>[2x]MASMKTAQE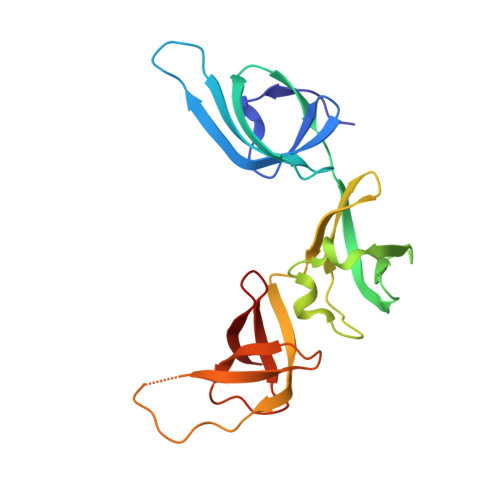FRAGQVANINGAPWVIQKAEFNKSGRNAAVVKMKLKNLLTGAGTETVFKADDKLEPIILDRKEVTYSYFADPLYVFMDSEFNQYEIEKDDLEGVLTFIEDGMTDICEAVFYNDKVISVELPTTIVRQIAYTEPAVRGDTSGKVMKTARLNNGAELQVSAFCEIGDSIEIDTRTGEYKSRVKA(2R)-1-[6-[(2R)-2-carboxypyrrolidin-1-yl]-6-oxidanylidene-hexanoyl]pyrrolidine-2-carboxylic acid | 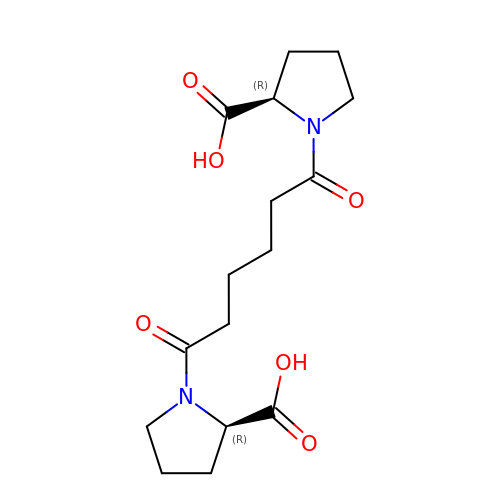C16 H24 N2 O6 | HZLAWYIBLZNRFZ-VXGBXAGGSA-N>[2x]MASMTGGQQMGRDEAGITGTWYNQLGSTFIVTAGADGALTGTYESAAGKAESRYVLTGRYDSAPATDGSGTALGWTVAWKNNYRN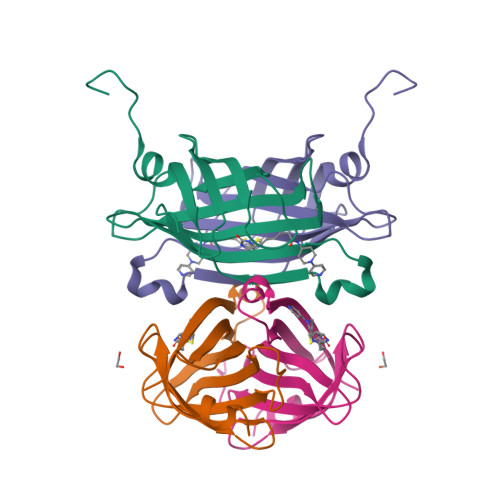AHSATTWSGQYVGGAEARINTQWLLTAGTTEANGWASTLVGHDTFTKVKPSAASIDAAKKAGVNNGNPLDAVQQ Class A plexins (PlxnAs) act as semaphorin receptors and control diverse aspects of nervous system development and plasticity, ranging from axon guidance and neuron migration to synaptic organization. Plexins are large type 1 transmembrane proteins comprising typically ten domains in their extracellular segment, a single membrane spanning region that is predicted to be helical and a conserved, cytoplasmic region that contains a GTPase-activating protein (GAP) domain with a Rho GTPase-binding domain insert. All our PlxnA ectodomain structures show autoinhibitory, intermolecular “head-to-stalk” (domain 1 to domain 4-5) interactions, which are confirmed by biophysical assays, live cell fluorescence microscopy, and cell-based and neuronal growth cone collapse assays. This work reveals a 2-fold role of the PlxnA ectodomains: imposing a pre-signaling autoinhibitory separation for the cytoplasmic domains via intermolecular head-to-stalk interactions and supporting dimerization-based PlxnA activation upon ligand binding.

We determined crystal structures of the full extracellular segments of mouse PlxnA1, PlxnA2, and PlxnA4 from eight crystal forms providing a total of 13 independent structures that range in maximum resolution from 4 to 10 Å. In five out of 13 full extracellular structures all ten domains are resolved whereas in the other eight structures some of the C-terminal domains were not modeled due to fragmentary or absent electron density. This indicates that some flexibility is present in the extracellular segment of plexins. Some flexibility in the stalk is evident on comparison of the 13 different structures and contributes to the ring diameter ranging from 84 Å to 99 Å. All our PlxnA full ectodomain crystal structures have an intermolecular plexin–plexin interface in common. This interface is formed by blades 1–3 of the sema domain of one plexin molecule and the outer side of domains 4-5 (PSI2-IPT2) from the ring of a second plexin. The residues in this interface are conserved among vertebrate PlxnAs but much less among all plexins, suggesting that this plexin–plexin interaction may be an important functional feature of PlxnAs.

>ETGKPSFVTFRGEPAEGFNHLVVDERTGHIYLGAVNRIYKLSSDLKVLVTHQTGPDEDNPKCYPPRIVQTCNEPLASTNNVNKMLLIDYKENRLIACGSLYQGICKLLRLEDLFKLGEPFHKKEHYLSGVNESGSVFGVIVSYSNFDDKLFIATAVDGKPEYFPTISSRKLTKNSEADGMFAYVFHDEFVASMIKIPSDTFTVIPDFDIYYVYGFSSGNFVYFLTLQPEMVSPPGSTTKEQVYTSKLVRLCKEDTAFNSYVEVPIGCERNGVEYRLLQAAYLSKAGAVLGRTLGVRPDDDLLFTVFSKGQKRKMKSLDESALCIFILKQINDRIKDRLQSCYRGEGTLDLAWLKVKDIPCSSALLTIDDNFCGLDMNAPLGVSEMVRGIPVFTEDRDRMTSVIAYVYKNHSLAFVGTKSGKLKKIRVDGPKGNALQYETVQVVDSGPVLRDMAFSKDHEQLYIMSERQLTRVPVESCGQYRSCGECLGSGDPHCGWCVLHNTCTRKERCERSREPRRFASEMKQCVRLTVHPNNISVSQYNVLLVLETYNVPELSAGVNCTFEDLSEMDGLVIGNQIQCYSPAAKEVPRIITENGDHHVVQLQLKSKETGMTFASTSFVFYNCSVHNSCLSCVESPYRCHWCKYRHVCTHDPNTCSFQEGRVKLPEDCPQLLRVDKILVPVEVIKPITLKAKNLPQPQSGQRGYECILNIQGIEQRVPALRFNSSSVQCQNTSYSYEGMEINNLPVELTVVWNGHFNIDNPAQNKVYLYKCGAMRESCGLCLKADPDFECGWCQSPGQCTLRQHCPAHESRWLELSGANSKCTNPRITEIIPVTGPREGGTKVTIRGENLGLEFRDIASHVKVAGVECSPLVDGYIPAEQIVCEMGEAKPSQHAGFVEICVAVCRPEFMARSSQLYYFMTLTLADLKPNRGPMSGGTQVTITGTNLNAGSNVVVMFGSQPCLFHRRSPSYIICNTTSSEEVLDMKVTVQVDRARIRQDLVFQYVEDPTIVRIEPEWSIVSGNTPIAVWGTHLDLIQNPQIRAKHGGKEHINICEVLNATEMTCQAPALALGPDHQSDLTERPEEFGFILDNVQSLLILNKTNFTYYPNPVFEAFSPSGILELKPGTPIILKGKNLIPPVAGGNVKLNYTVLVGEKPCTVTVSDVQLLCESPNLIGRHKVMARVGGMEYSPGMVYIAPGRTKHHHHHH[2x]> QDADKLPHTKVTLVAPPQVHPHEQATKSGPKVVEFTMTIEEKKMVIDDKGTTLQAMTFNGSMPGPTLVVHEGDYVQLTLVNPATNAMPHNVDFHGATGALGGAKLTNVNPGEQATLRFKADRSGTFVYHCAPEGMVPWHVVSGMSGTLMVLPRDGLKDPQGKPLHYDRAYT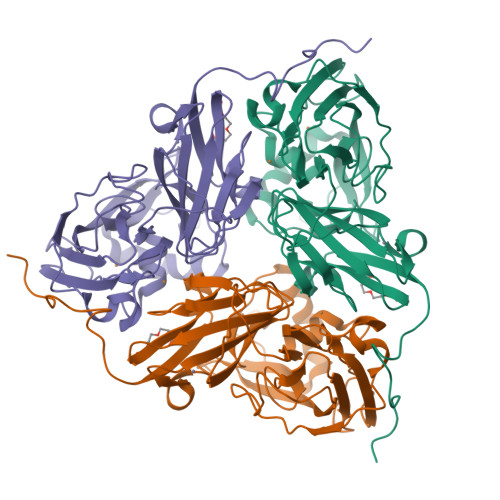IGEFDLYIPKGPDGKYKDYATLAESYGDTVQVMRTLTPSHIVFNGKVGALTGANALTAKVGETVLLIHSQANRDTRPHLIGGHGDWVWETGKFANPPQRDLETWFIRGGSAGAALYTFKQPGVYAYLNHNLIEAFELGAAGHIKVEGKWNDDLMKQIKAPAPIPR>GSMAEPLKEEDGEDGSAEPPGPVKAEPAHTAASVAAKNLALLKARSFDVTFDVGDEYEIIETIGNGAYGVVSSARRRLTGQQVAIKKIPNAFDVVTNAKRTLRELKILKHFKHDNIIAIKDILRPTVPYGEFKSVYVVLDLMESDLHQIIHSSQPLTLEHVRYFLYQLLRGLKYMHSAQVIHRDLKPSNLLVNENCELKIGDFGMARGLCTSPAEHQYFMTEYVATRWYRAPELMLSLHEYTQAIDLWSVGCIFGEMLARR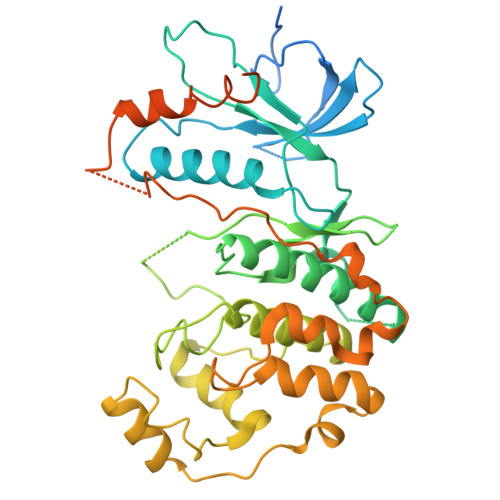QLFPGKNYVHQLQLIMMVLGTPSPAVIQAVGAERVRAYIQSLPPRQPVPWETVYPGADRQALSLLGRMLRFEPSARISAAAALRHPFLAKYHDPDDEPDCAPPFDFAFDREALTRERIKEAIVAEIEDFHARREGIRQQIRFQPSLQPVASEPGCPDVEMPSPWAPSGDCAMSGRHHHHHH[2x]> DHGSENGWPKHTACNSGGLEVVYQSCDPLQDFGLSIDQCSKQIQSNLNIRFGIILRQDIRKLFLDITLMAKGSSILNYSYPLCEEDQPKFSFCGRRKGEQIYYAGPVNNPGLDVPQGEYQLLLELYNENRATV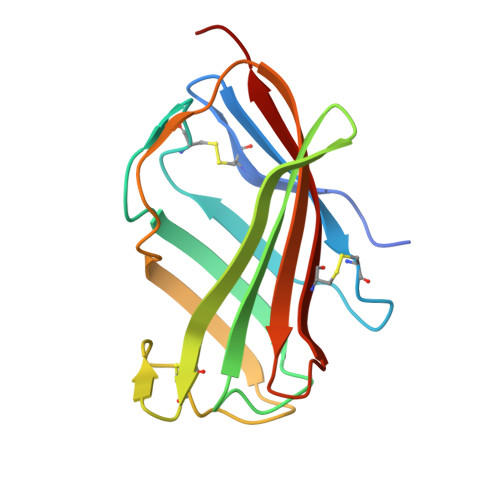ACANATVTSSEF>MKLIFAIVQDQDSNRLSDALTKGNFGATKLATTGGFLKAGNTTFIIGTEDERVEDALAIIKENCKAREQMMTPSASLGVTVDTYVPYPIEVQVGGATVFVMPVESFHHFLEHH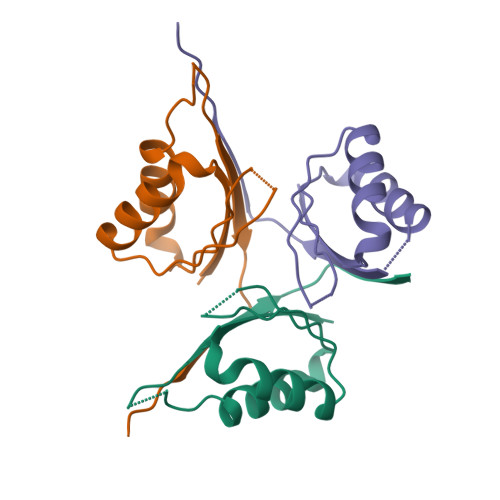H[3x]>GSHMSTPARRRLMRDFKRMKEDSPPGVSASPLPDNVMIWNAMIIGPADTPYEDGTFRLLLEFDEEYPNKPPHVKF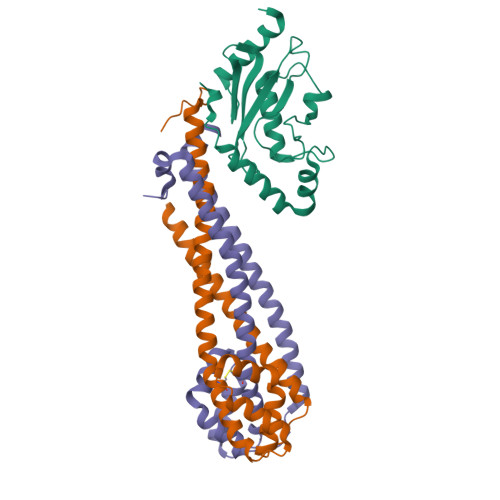LSEMFHPNVYANGEICLDILQNRWTPTYDVASILTSIQSLFNDPNPASPANVEAATLFQDHKSQYVKRVKETVEKSWEDDMEDMADEDEDEE[2x];>[4x]MNDHFVKRPKLELSDPSEPLTQKDVIAFQKEALFRCLNKWRVKANQLVEENEVLAAGLSKTTESVSGCCSSIVVLARSVVEDCSDEQDKRFLQQLINTEDEHTLTQIISNNSARICELILKTSGSNISDNIGRLQELESLTLTLQKLLKSSENKLKKATEYYENIIAQYDRQDSESVSRVFNTADDDSNVKKEKQSSTGASSVNDE>[2x]MLTIDYNSYRTTTPYGKRVRFLVLHYTALDFAASVKALTTGAASAHYLIPAPHDPSYKAAGFKGQRIFNLVAEE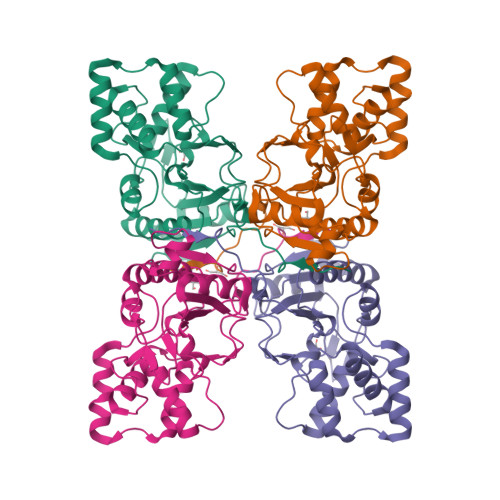DRAWHAGVSGWARRDNLNDTSIGIEIVNLARDDDGVFTFPDYERSQINALKQLAKNILQRYPDMTPKNVVGHSDIAVGRKSDPGPKLPWKELYEAGIGAWYDDATRDRYREGFERDGLPPRADLLEAFRLYGYALPATVDDAYFASLLRAFQMHFRPENYDGALDVETAAILYALNEKYPA> VSSPVST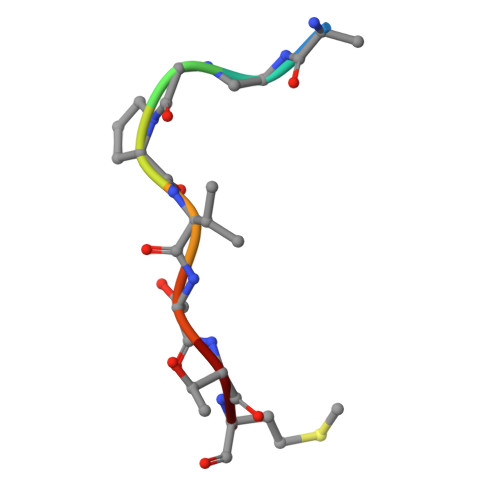M> NELNN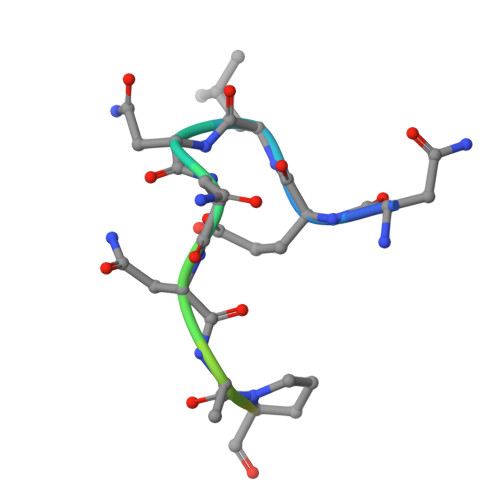NLPGGAPAAP DdPoxB belongs to class B of the family of so-called dye-decolorizing peroxidases, whereas DdPoxA is a member of the peroxidase–cyclooxygenase superfamily. Phylogenetic analysis demonstrated that DdPoxA belongs to family 6 of this heme peroxidase superfamily, shares a striking sequence similarity to the mammalian heme peroxidases, and has a signal peptide for secretion. The metalloenzyme is shown to follow the halogenation cycle and to catalyze the efficient two-electron oxidation of iodide and thiocyanate. Summing up, in this report we present the first structural and functional characterization of a heme peroxidase with one heme to protein ester bond. Its high efficiency in H2O2-dependent iodide and thiocyanate oxidation and its expression at multicellular lifestyle of D. discoideum together with its antibacterial activity suggest that this secreted and highly stable glycoprotein acts in the first line defense of the fruiting bodies containing spores against bacteria.

The structure was solved to 2.5 Å resolution by molecular replacement using the balbes web server. Fig. 4A shows the overall largely α-helical structural organization of DdPoxA. The protein is composed of 21 α-helices of varying length. The central core of the molecule consists of five long α-helices (H2, H6, H7, H8, and H13) with the covalently attached heme group. The conserved distal residues Gln-97 and His-101 are found in helix 2, whereas the proximal His-325 belongs to helix 8 and the proximal Asn-403 and Arg-406 are part of helix 13. The important catalytic residues on the distal heme site (His-101, Gln-97, and Arg-233) are fully conserved, including Glu-236 that forms an ester bond with the 1-methyl substituent of the heme porphyrin ring. However, DdPoxA lacks the covalent ester bond that is formed between the heme and the distal aspartate in LPO, because the corresponding residue in DdPoxA is an isoleucine. In LPO, the Ca2+-binding site consists of the residues Asp, Asp, Ser, Tyr, and Phe, and in DdPoxA, the ion is coordinated by Asn-102, Gly-167, Tyr-169, Asp-171, and Asn-173. The polypeptide chain of DdPoxA contains eight cysteines, six of which are involved in disulfide bridges (Cys-120–Cys-128, Cys-146–Cys-159, and Cys-277–Cys-505). However, in the crystal structure, only one GlcNAc is left on each N-glycosylation site due to the deglycosylation procedure.

>SQEFRSYTGEGNNKQNPKQGSIFTPFIRLANPIKFNKNGFPNITNQPSRAISNIIFDQQTHIGSKEHLTDMFNMWGQFLIHNMALSKPEPNSWPIKVPKCDQYFDPACIGNKTMNYFRTRATEVPCDVGKTVVDEDGKCYEQINSLGSYIDGNVLYGNSEEICKNLRSLSGGEMKMTVTDVGDLPPKNVPGVPMDNDANLFPIDQLYSVGERRGNENPGLLSIHTLLLRDHNRLARKFARLHPEWDDERVFQQSRSCIIEQIQKITYDEYLPTTLGSFPSYTGYDANVNAQVSNEFTTTAFRFGHSEVGPFMEYYSENGTRLQPLPIKFSYFNPHALNRGVEPLIRGLIINEEENIDIYMISDLRNFLFGKPGQGGLDLASRNLQRNRDHGIPPYNSLRRQLGLRPVQTWSDITSDPQIQNRLKNAYKSVDDIDSYVGGLAEDHMEGSCVGQTFYLIIYEQFFRTRAGDRFWYETPEMRMVNRECETTTFAEVIKRTTSNIGYVQPNVFRK[2x]>MRKEAIYHRPADNFAYAYDSETLHLRLRTKKDDIDRVELLHGDPYDWQNGAWQFQMMPMRKTGSDELFDYWFAEVKPPYRRLRYGFVLYSGEEKLVYTEKGFYFEVPTDDTAYYFCFPFLHRVDLFEAPDWVKDTVWYQIFPERFANGNPSISPEGSRPWGSEDPTPTSFFGGDLQGIIDHLDYLVDLGITGIYLTPIFRSPSNHKYDTADYFEVDPHFGDKETLKTLI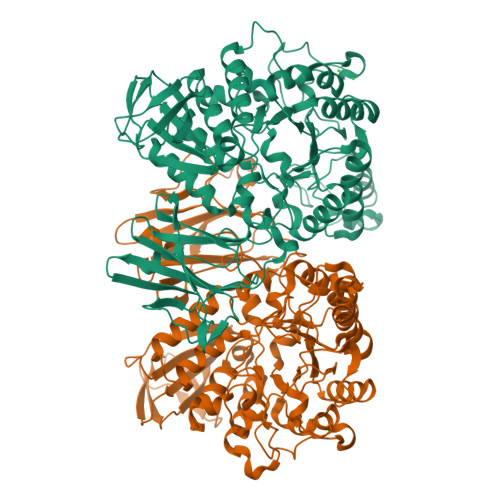DRCHEKGIRVMLDAVFNHCGYEFAPFQDVWKNGESSKYKDWFHIHEFPLQTEPRPNYDTFAFVPQMPKLNTANPEVKRYLLDVATYWIREFDIDGWRLDVANEIDHEFWREFRQEVKALKPDVYILGEIWHDAMPWLRGDQFDAVMNYPFTDGVLRFFAKEEISARQFANQMMHVLHSYPNNVNEAAFNLLGSHDTSRILTVCGGDIRKVKLLFLFQLTFTGSPCIYYGDEIGMTGGNDPECRKCMVWDPMQQNKELHQHVKQLIALRKQYRSLRRGEISFLHADDEMNYLIYKKTDGDETVLVIINRSDQKADIPIPLDARGTWLVNLLTGERFAAEAETLCTSLPPYGFVLYAIEHW[2x]>[8x]SNAQEQRM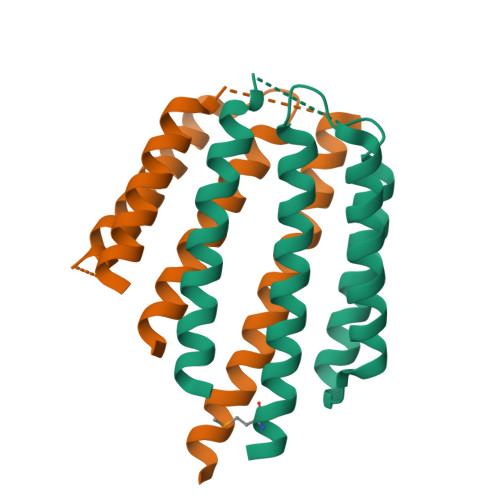SHHYATIEVSQQLRQLLGDQLVILLRETPDGQALERSQNDFRRVLEQGRANTVDSAEQAALDGVRDAYLQLQAHTPALLEAPMADNDGFSEAFNGLRLRLQDLQQLALAGISEAETSARHRA> SDTAPAGFQLEKVVILSRHGVRAPTKMTQTMRDVTPHQWPEWPVKLGYITPRGEHLISLMGGFYRERFQQQGLLPKDNCPTPDAVYVWADVDQRTRKTGEAFLAGLAPQCDLAIHHQQNTQQADPLFHPVKAGICSMDKSQVHAAVEKQAGTPIETLNQRYQASLALMSSVLDFPKSPYCQQHNIGKLCDFSQAMPSRLAINDDGNKVALEGAVGLASTLAEIFLLEHAQGMPKVAWGNIHTEQQWNSLLKLHNAQFDLMSRTPYIAKHNGTPLLQTIAHALGSNITSRPLPDISPDNKILFIAGHDANIANISGMLGMTWTLPGQPDNTPPGGALVFERWVDNAGKPYVSVNMVYQTLAQLHDQAPLTLQHPAGSVRLNIPGCS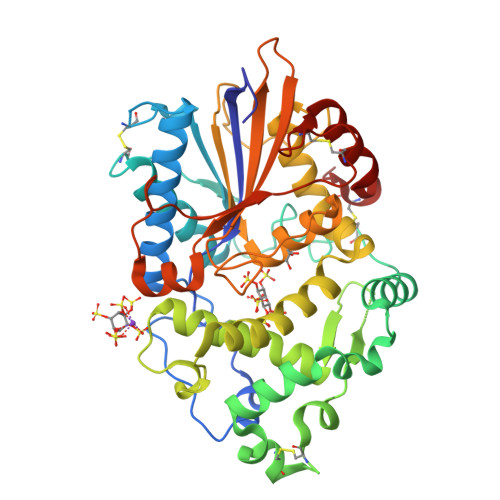DQTPDGYCPLSTFSRLVSHSVEPACQLP Dimethyl 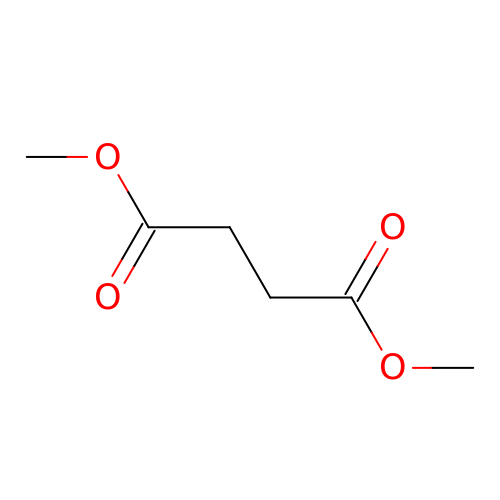fumarate | C6 H10 O4 | MUXOBHXGJLMRAB-UHFFFAOYSA-N> MEEDIAYVKDLVSKYLVDNERLSRQKLAFLVQTEPRMLLMEGLKLLSLCIEVDSCNANGCEHNSEDKSVEKILHECGILTPSLCFVVPDGYKLTGNVLILLECFVRSSPANFEQKYIEDLKKLEQLREDLKSVDINLIPLIDGRTSFYNEQLPDWVNDKLRDTLFSLLRYAQESNSLFEESEYSRLCESLSMTSGRLSGIESLNTLLDNRSDHYEEIIALCHQGINNKLTAHEVKLQIEEEYQVFRNRLRGGEIKCQFMRVNKDHLLSEFNKLYIDDGVVVEENLEQLTHQFKRASPILRFLYSDIEGEEDRRNTQAIKEHQMQCWRSFLNKVKSLRILNTRRKLLLIFDTLILLASKYDHIKQGCLQGWLGSCFVSVNDRLVSLDSTKRDLKKWIERRQQVESSKSTAPSQCLSKNQILSSIIQKTIKRATAAMEDVGINMNHFGVDMSVIGLDCYDSIMNFDVTGVTPTISYQKSQEETFPYAMGVVELSETTDLGRLSSLSLALINSMKTSSTVKLRQNEFGAARYQVVRCKEAYCQEFLLDGVKFQLVYQKTGECSKCYAINNDKVGEVCSFYADPKRYFPAIFSAEVLQATVDTMITWIKDCNELEKELTHIKLLTKMILVLILAHPSKRSQKLLQNLRYFIMAYVSDYHHVDLMDKIKEKLITETEFLLYKLIRALISLILCNEVKSMMTNRFKFILNVSYMCHFITKETPDRLTDQIKCFEKFLEPKIEFGHVSVNPADIATEEELMDMAYHAKKFLSKEGCTAPRGPEYKKPGVSKKFLSLLTSSFNNGSLFKEKEVKKELRDPIITSGCATALDLASNKSVVVNKYTDGSRVLNYDFNKLTALAVTQLTEVFSRKGKHLLNRQDYEYKVQQAMSNLVLGSQQQGVNVDRSDLDEILLEGSASLYFDQLRETVQKIVDQYREPAGLGSMKGGNSEPSINDLDELIPNKFHIRLIKGELSNHMVEDFDCEILPDSFYKEFCDNVYSNHKMKEKYFYCGHMSQCPIGELSKAVTTRTYFEQEYFQCFKSVLLIMNANKLMGKYSHYRSRNLNFKFDTGKLSDDVRISERESNSEALSKALSLTNCTTAMLKNLCFYSQESPQSYNSVGPDTGRLKFSLSYKEQVGGNRELYIGDLRTKMFTRLIEDYFEALSLQLSGSCLNNEKEFENAILSMKLNVSLAHVSYSMDHSKWGPMMCPFLFLAVLQNLIFLSKDLQADIKGRDYLSTLLTWHMHKMVEIPFNVVSAMMKSFIKAQLGLRKSTSQSITEDFFYSNFQVGVVPSHVSSILDMGQGILHNTSDFYALISERFINYAISSVCGGSIDAYTSSDDQISLFNQDLTDLMQRDPEEFKTLLEFHYYMSNQLNKFISPKSVVGRFVAEFKSRFYVWGDEVPLLTKFVAAALHNIKCKEPHQLAETIDTIIDQSVANGVPVHLCNLIQLRTLSLLQYARYPIDPFLLNCETDVKDWVDGNRSYRIMRQIESLIPEACGKIRSMLRKLFNKLKTGQLHEEFTTNYLSGEHVSSLKNLCIILDVDPPSESDLEFSWLNLAAYHPLRMVLRQKVIYSGAVNLDDEKIPTIVKTIQNKLSSTFTRGAQKLLSEAINKSAFQSSIASGFVGLCRTLGSKCVRGPNKENLYIKSIQSLISNTQGIELLTNNHGIQYWRVPLNLKEEKISVAGYFRPLLWDYMCISLSTAIELGAWVLGEPKAAKPLEFFKHNPCDYFPLKPTASKLLEDRVGVNHIIHSLRRLYPSMFEKHILPFMSDLASTKMKWSPRIKFLDLCVALDVNCEALSLVSHIVKWKREEHYIVLSSELRLSHSRSHEPMVEERVVSTSDAVDNFMRQIYFE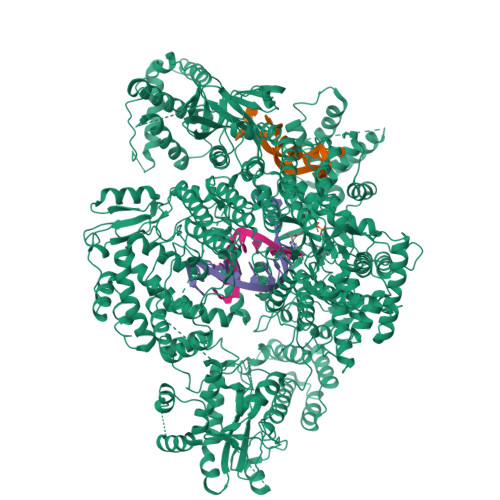SYVRSFVATTRTLGSFTWFPHKTSIPEGEGLQRLGPFSSFVEKVIYKGIERPMFKYDLMMGYAWIDFDVEPAKFNYNQLIASGLVSSKFDSLEDFFDAIESLPPGSVKLSQTIRFQIKSQDASFRESFAIHLNFVGSMNEQGKYLVQDVAVMYSGAVNSCVLTDCWRLVLSGPTFKGKSAWYVDTEAINEFMSDTNQLGEVTPVEIVIDIDRLQFVEHDFVLVGPCSEAIPLVVHRGGLWECNKRLASFSPVLQDQDLELFVREVGDTSPDLLIGALSAMMLDRLKLRMQWSGVDIVSVLKKVMPKDGLKVLNAAFEAVDDWIEFKGYALCFSKSKRRVMIQSSGGKLRLKGRTCEELLEKEEEVEDIESASNSLEVLFQ Based on a literature survey and a preliminary activity screen of heterologously expressed potential para‐carboxylases, 3,4‐dihydroxybenzoic acid decarboxylases from Enterobacter cloacae (EcAroY) and Klebsiella pneumoniae (KpAroY, 89 % identical) were selected for further studies.2d, 13 Both enzymes belong to the UbiD family and are related to a ferulic acid decarboxylase (Fdc1), which has been shown to facilitate the (de)carboxylation of cinnamic acids in the presence of a recently discovered prenylated flavin (prFMN) cofactor. The AroY monomer consists of an N‐terminal prFMN‐binding domain (residues 1–339), an oligomerization domain (residues 340–475), and a C‐terminal α‐helix (residues 476–495). A comparison with the previously reported structures of the fungal Fdc1 and E. coli UbiD14 shows that AroY structures adopt an “open” conformation, where the position of the prFMN domain is more akin to that observed for UbiD, compared to the more closed conformation observed for Fdc1. Crystal structures and in vitro reconstitution data unambiguously demonstrate that prFMN is employed as a cofactor, and that oxidative maturation is required for activity.

However, upon purification of the decarboxylase from the E. coli host, only little enzyme activity could be detected for either of the two enzymes, despite additional co‐expression with the UbiD‐associated prenyltransferase UbiX to provide sufficient prFMN in vivo. A comparison of the KpAroY and EcAroY crystal structures revealed only small differences, in accordance with the similar activities observed in solution experiments.

>[2x]MQNPINDLRSAIALLQRHPGHYIETDHPVDPNAELAGVYRHIGAGGTVKRPTRTGPAMMFNSVKGYPGSRILVGMHASRERAALLLGCVPSKLAQHVGQAVKNPVAPVVVPASQAPCQEQVFYADDPDFDLRKLLPAPTNTPIDAGPFFCLGLVLASDPEDTSLTDVTIHRLCVQERDELSMFLAAGRHIEVFRKKAEAAGKPLPVTINMGLDPAIYIGACFEAPTTPFGYNELGVAGALRQQPVELVQGVAVKEKAIARAEIIIEGELLPGVRVREDQHTNTGHAMPEFPGYCGEANPSLPVIKVKAVTMRNHAILQTLVGPGEEHTTLAGLPTEASIRNAVEEAIPGFLQNVYAHTAGGGKFLGILQVKKRQPSDEGRQGQAALIALATYSELKNIILVDEDVDIFDSDDILWAMTTRMQGDVSITTLPGIRGHQLDPSQSPDYSTSIRGNGISCKTIFDCTVPWALKARFERAPFMEVDPTPWAPELFSDKK>[2x]MKHHHHHHPMTTKQWGITPPISTAPATEQENALNTALINELKNQNLFESPAESEKRVKVLDELQQITTEFVKKVSLAKHMNEKMANEAGGKIFTYGSYRLGVYGPGSDIDTLVVVPKHVSRDNFFQDLEPMLREREEVTDLAAVPDAYVPIIKFKFLGISIDLIFARLSVPRVPRDLELSDNNLLKGVEERCVLSLNGTRVTDQILQLVPNRAVFKHALRAIKFWAQRRAIYANVVGFPGGVAWAMMVARICQLYPNAVSSVIVAKFFRILHQWNWPQPILLKPIEDGPLQVRIWNPKLYPSDKAHRMPIITPAYPSMCATHNITLSTQTIILREMVRAGEIADQIMVKALPWSALFQKHDFFHRYKHYLTITAAAKTAEAQLKWAGLVESKLRHLVTRLELVDAIALAHPFNKGFDKVYNCSSEEEAQQVASGVTLEVAYESTDHEKLANDTVNEEKADNTESKADGSENGEKQIFPVYTTTCYIGLELEKKKGHPIKRLDISWPTQEFYELCKKWDKYDDTLMNVFIKNTKNTALPDEVFEPGEERPKATKKRSTADTAHSTEQLKRQKVSTA;>[2x]GAMGISLPLLKQDDWLSSSKPFGSSTPNVVIEFDSDDDGDDFSNSKIEQSNLEKPPSNSENGGSHHHHHH

The S. pombe orthologue of the human PAXT connection, Mtl1-Red1 Core (MTREC), is an eleven-subunit complex that targets cryptic unstable transcripts (CUTs) to the nuclear RNA exosome for degradation. It encompasses the canonical poly(A) polymerase Pla1, responsible for polyadenylation of nascent RNA transcripts as part of the cleavage and polyadenylation factor (CPF/CPSF). We report crystal structures of Pla1 in its apo form and in complex with Red1. Taken together, our data reveal the molecular details of recruitment of Pla1 by Red1 which leads to hyperadenylation of CUTs, serving as a signal for exosome-mediated target degradation.

To understand the molecular details of the Red1-Pla1 interaction, we determined the crystal structure of the complex. Co-crystals of the complex appeared within three weeks and diffracted to 2.81 Å resolution. The asymmetric unit contains two molecules of the Pla1-Red1 heterodimer which exhibit small differences between them, as indicated by a root mean square deviation (RMSD) of 0.96 Å. Our crystal structure of the Pla1-Red1 complex shows that Red1 contacts the C-terminal RRM domain of Pla1. The interaction between Pla1 and Red1 buries a total solvent accessible area of 1338.5 Å2. The interaction interface of Red1 can be largely divided into two regions. The first half comprises a short α-helix at the N-terminus (α0) that helps orient Red1 onto Pla1. A network of aromatic stacking interactions occurs between Pla1RRM Phe468 and Red1 Trp298 and Phe305. The second half of Red1 is largely involved in mainchain-sidechain interactions between Red1 residues Gly306, Ser308, Asn311 and Val312 that pack against Pla1 residues Gln420, Val518, Ile520 and Asn522. In addition to these, the Red1 C-terminus, spanning residues 323–345, is flexible and therefore not observed in the crystal structure of the complex.> MGWSLPKEKGLILCLWNKFCRWFHRRESWAQSRDEQNLLQQKRIWESPLLLAAKENNVQALYKLLKFEGCEVHQKGAMGETALHIAALYDNNEAAQVLMEAAPELVFEPMTSELYEGQTALHIAVINQNVNLVRALLARGASVSARATGSVFHYRPHNLIYYGEHPLSFAACVGSEEIVRLLIEHGADIRAQDSLGNTVLHILILQPNKTFACQMYNLLLSYDGGDHLKSLELVPNNQGLTPFKLAGVEGNIVMFQHLMQKRKHIQWTYGPLTSTLYDLTEIDSSGDDQSLLELIVTTKKREARQILDQTPVKELVSLKWKRYGRPYFCVLGAIYVLYIICFTMCCVYRPLKPRITNRTNPRDNTLLQQKLLQEAYVTPKDDLRLVGELVSIVGAVIILLVEIPDIFRLGVTRFFGQTILGGPFHVIIVTYAFMVLVTMVMRLTNSDGEVVPMSFALVLGWCNVMYFARGFQMLGPFTIMIQKMIFGDLMRFCWLMAVVILGFASAFYIIFQTEDPDELGHFYDYPMALFSTFELFLTIIDGPANYDVDLPFMYSITYAAFAIIATLLMLNLLIAMMGDTHWRVAHERDELWRAQVVATTVMLERKLPRCLWPRSGICGREYGLGDRWFLRVEDRQDLNRQRIRRYAQAFQQQDDLYSEDLEKDSGEKLVPRLVPR

TRPV6 and its close relative TRPV5 are TRP channels that are distinctly Ca2+-selective and play an important role in calcium homeostasis. Structurally, TRP channels are assemblies of four identical subunits arranged symmetrically around the pore axis. The transmembrane domain of TRP channels includes six transmembrane helices (S1–S6) and a pore loop (P-loop) between S5 and S6. S5, P-loop and S6 form the KcsA channel-like pore domain, with the ion conduction pathway lined by the S6 helices and extracellular loops connecting the P-loop helix to S5 and S6.

TRPV6* crystallized in a nearly identical crystal lattice to TRPV6cryst and the overall shape of the molecule was very similar. Despite these similarities, to our great surprise, the structure of TRPV6* exhibited the domain swapped fold observed in other TRP channels of known structure. Therefore, the crystallographic data unambiguously demonstrates that the TRPV6* structure is domain-swapped. Apart from the distinct connectivity between S4 and S5 as well as S6 and TRP helix, the domain-swapped TRPV6* and non-swapped TRPV6cryst structures were almost identical. Similarly, both the 2Fo-Fc and robust Fo-Fc omit maps for TRPV6* demonstrated completely different connectivity of transmembrane domains compared to TRPV6cryst. In TRPV6*, L495 projects its side chain into a hydrophobic pocket formed by residues of S5 and S6 of one subunit and residues at the S4–S5 elbow of the adjacent subunit. By contrast, in TRPV6cryst, Q495 is rotated by ~120° with respect to the orientation of L495 in TRPV6* and forms polar interactions with the hydrophilic pocket formed by S4–S6 and the TRP helix of the same subunit. These observations suggest that hydrophobic burial of the L495 residue plays an important role in driving the domain-swapped fold of TRPV6. Despite these gross similarities, kinetic analysis indicated the rate of increase in Fura-2 signal is faster in TRPV6* compared to TRPV6cryst.> MMSLDIQCEQLSDARWTELLPLIQQYEVVRLDDCGLTEVRCKDISSAVQANPALTELSLRTNELGDGGVGLVLQGLQNPTCKIQKLSLQNCGLTEAGCGILPGMLRSLSTLRELHLNDNPMGDAGLKLLCEGLQDPQCRLEKLQLEYCNLTATSCEPLASVLRVKADFKELVLSNNDLHEPGVRILCQGLKDSACQLESLKLENCGITAANCKDLCDVVASKASLQELDLSSNKLGNAGIAALCPGLLLPSCKLRTLWLWECDITAEGCKDLCRVLRAKQSLKELSLASNELKDEGARLLCESLLEPGCQLESLWIKTCSLTAASCPYFCSVLTKSRSLLELQMSSNPLGDEGVQELCKALSQPDTVLRELWLGDCDVTNSGCSSLANVLLANRSLRELDLSN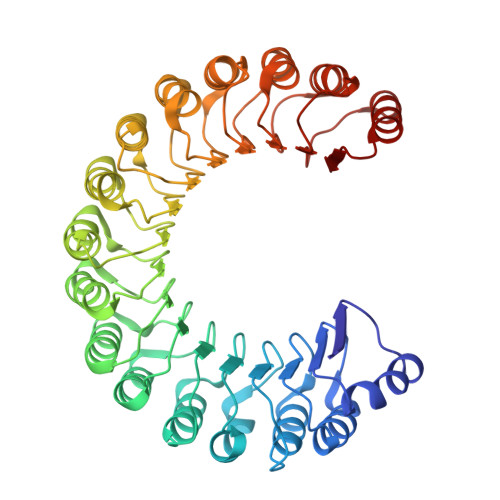NCMGGPGVLQLLESLKQPSCTLQQLVLYDIYWTNEVEEQLRALEEERPSLRIIS>MIDLNIMKVANYINGEFKEPSTGAFQVKTSPVDGSKIAEVPRSGREDAREAIDSAFEALKAWANIPAIRRAEYLYKMLEVFRQMKEDFMKILTVEGGGTYRKVWGEVVFTERLIQNAAELARHYQGRVLQSDSESTISVVFKRSKGVVGVITPWNYPLSISMKKIAHTLAVGNTVVYKPASDTPVTGWLIAQMVAKAGLPKGVFNLVIGPGPVVGEEIVTHKRVAHVTFTGESSTGREIAAKAAGTLKTVTLELGGSDPLIILDDVDVDYAARLAVFASLFHQGQICTSAKRIIVHKAVADKFIERYVHYVKMLRIDDPRKDEKVDLGPLINERQVALMKEFVDDAVSRGGRLLIGGRSWGNFFEPAIFVDVDRNFRIMREEVFGPVRPIVVVENDDQAVEVANDTDYGLSGAVLTNNVNRAFRIAEAVESGMFHINDVTFLEESHVPFGGIKASGVGREGGEWSFHETTYDRWVTVTLRTRRFPIPSALK[8x]

In the present work, we report the structural and functional characterization of the first thermostable archaeal dehydrogenase (AlDHPyr1147). The kinetic data showed that AlDHPyr1147 is strictly specific for NADP+ and is active with aliphatic aldehydes. According to gel filtration, AlDHPyr1147 is a tetramer. The AlDHPyr1147 subunit consists of three domains: the coenzyme-binding domain (residues 1–256, 443–470), the catalytic domain (residues 257–442), and the oligomerization domain (residues 122–144, 470–491).

The crystal of Holo-2 was grown by cocrystallization of the apo form with NADP+, whereas the crystal of Holo-3 was prepared by soaking crystals of the apo form in a solution of NADP+ and isobutyraldehyde. In Holo-2, the conformations of the coenzyme and the active site residues are very similar to those in the Holo-1 structure. The main difference is in the conformation of Glu253. In Holo-2, Glu253 has two conformations, the “inside” and “intermediate” conformations. In the latter conformation, the γ-carboxyl group of Glu253 is directed away from the active site and is at a distance of 2.7 Ǻ from O_Phe449. In this conformation, Glu253 is not involved in a hydrogen bond with nitrogen of Gly255, and the carbonyl oxygen of Leu254 is rotated by 180°. It should be noted that, as follows from the crystallization conditions for the Holo-2 structure, the coenzyme is in the oxidized form. While the nicotinamide part of the coenzyme is flexible and adopts different conformations, the adenine part of the coenzyme is well ordered in all complexes of AlDHPyr1147. The adenine part of the coenzyme is fixed in a narrow cleft between helix 211–230 and helix 230–244; the 5′-phosphate of the adenosine ribose forms hydrogen bonds with Lys178, Ser181, and Gly211.9-hex-5-ynylpurin-6-amine | C11 H13 N5 | 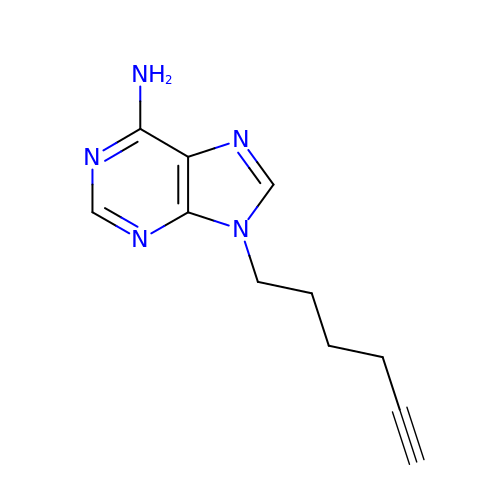VJWZTRUHTCSPRU-UHFFFAOYSA-N>[2x]MASEFTLMPMLITNPHLPDNPIVFANPAFLKLTGYEADEVMGRNCRF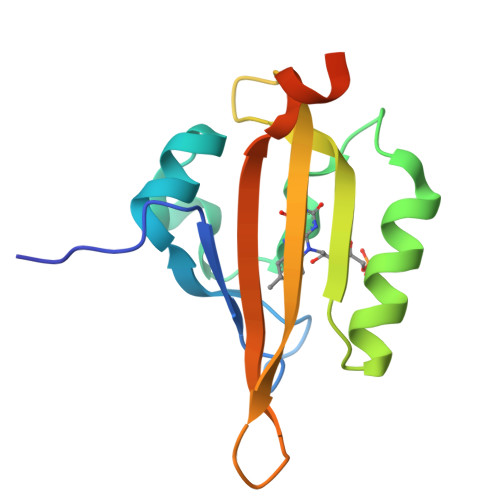LQGHGTDPAHVRAIKSAIAAEKPIDIDIINYKKSGEAFWNRLHISPVHNANGRLQHFVSSQLDVTLELVPRGSLEHHHHHH> MLVFIDDGSTNIKLQWQESDGTIKQHISPNSFKREWAVSFGDKKVFNYTLNGEQYSFDPISPDAVVTTNIAWQYSDVNVVAVHHALLTSGLPVSEVDIVCTLPLTEYYDRNNQPNTENIERKKANFRKKITLNGGDTFTIKDVKVMPESIPAGYEVLQELDELDSLLIIDLGGTTLDISQVMGKLSGISKIYGDS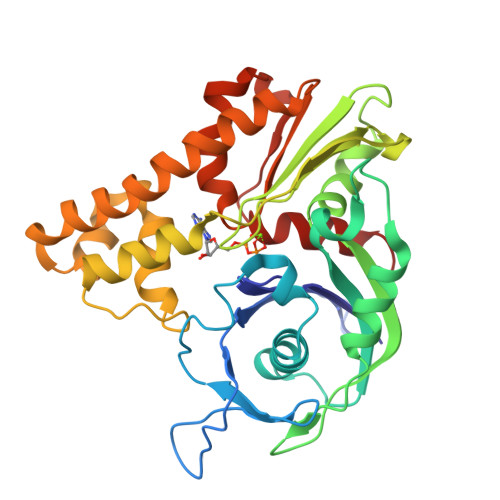SLGVSLVTSAVKDALSLARTKGSSYLADDIIIHRKDNNYLKQRINDENKISIVTEAMNEALRKLEQRVLNTLNEFSGYTHVMVIGGGAELICDAVKKHTQIRDERFFKTNNSQYDLVNGMYLIGN>MEHKRGHVLAVPYPSQGHITPFRQFCKRLHFKGLKTTLALTTFVFNSINPDLSGPISIATISDGYDHGGFETADSIDDYLKDFKTSGSKTIADIIQKHQTSDNPITCIVYDAFLPWALDVAR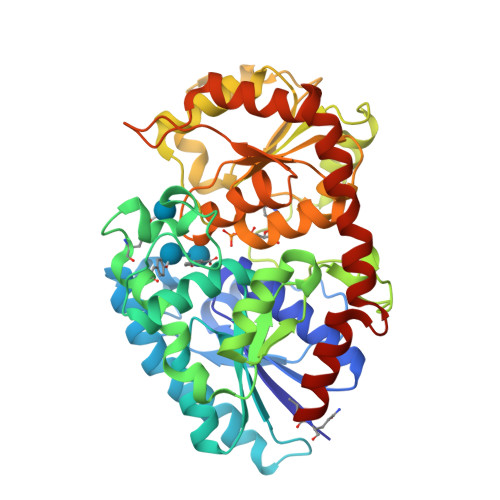EFGLVATPFFTQPCAVNYVYYLSYINNGSLQLPIEELPFLELQDLPSFFSVSGSYPAYFEMVLQQFINFEKADFVLVNSFQELELHENELWSKACPVLTIGPTIPSIYLDQRIKSDTGYDLNLFESKDDSFCINWLDTRPQGSVVYVAFGSMAQLTNVQMEELASAVSNFSFLWVVRSSEEEKLPSGFLETVNKEKSLVLKWSPQLQVLSNKAIGCFLTHCGWNSTMEALTFGVPMVAMPQWTDQPMNAKYIQDVWKAGVRVKTEKESGIAKREEIEFSIKEVMEGERSKEMKKNVKKWRDLAVKSLNEGGSTDTNIDTFVSRVQSK[2x]> ETPPRFTRTPVDQTGVSGGVASFICQATGDPRPKIVWNKKGKKVSNQRFEVIEFDDGSGSVLRIQPLRTPRDEAIYECVASNNVGEISVSTRLTVLREDQIPRGFPTIDMGPQLKVVERTRTATMLCAASGNPDPEITWFKDFLPVDTSNNNGRIKQLRSESIGGTPIRGALQIEQSEESDQGKYECVATNSAGTRYSAPANLYVRELREVRRVPPRFSIPPTNHEIMPGGSVNITCVAVGSPMPYVKWMLGAEDLTPEDDMPIGRNVLELNDVRQSANY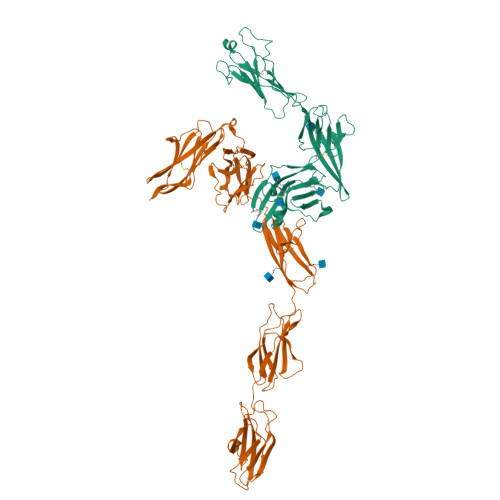TCVAMSTLGVIEAIAQITVKALPKPPGTPVVTESTATSITLTWDSGNPEPVSYYIIQHKPKNSEEPYKEIDGIATTRYSVAGLSPYSDYEFRVVAVNNIGRGPASEPVLTQTSEQAPSSAPRDVQARMLSSTTILVQWKEPEEPNGQIQGYRVYYTMDPTQHVNNWMKHNVADSQITTIGNLVPQKTYSVKVLAFTSIGDGPLSSDIQVIT;> SERCDDWGLDTMRQIQVFEDEPARIKCPLFEHFLKYNYSTAHSSGLTLIWYWTRQDRDLEEPINFRLPENRISKEKDVLWFRPTLLNDTGNYTCMLRNTTYCSKVAFPLEVVQKDSCFNSAMRFPVHKMYIEHGIHKITCPNVDGYFPSSVKPSVTWYKGCTEIVDFHNVLPEGMNLSFFIPLVSNNGNYTCVVTYPENGRLFHLTRTVTVKVVGSPKDALPPQIYSPNDRVVYEKEPGEELVIPCKVYFSFIMDSHNEVWWTIDGKKPDDVTVDITINESVSYSSTEDETRTQILSIKKVTPEDLRRNYVCHARNTKGEAEQAAKVKQKVAAHHHHHH>[2x]LPDSVDWREKGCVTEVKYQGSCGACWAFSAVGALEAQLKLKTGKLVSLSAQNLVDCSTEKYGNKGCNGGFMTTAFQYI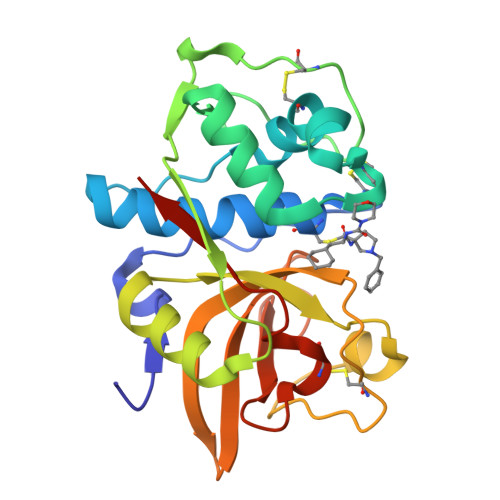IDNKGIDSDASYPYKAMDQKCQYDSKYRAATCSKYTELPYGREDVLKEAVANKGPVSVGVDARHPSFFLYRSGVYYEPSCTQNVNHGVLVVGYGDLNGKEYWLVKNSWGHNFGEEGYIRMARNKGNHCGIASFPSYPEIHHHHH>[6x]MFGYFYNSSFRRYATLMGDLFSNIQIKRQ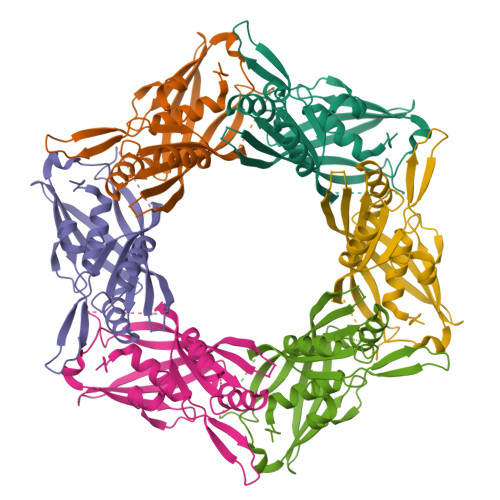LESGDKFIRVPITYASKEHFMMKLNKWTSINSQEDVAKVETILPRINLHLVDFSYNAPFKTNILNQNLLQKGATSVVSQYNPSPIKMIYELSIFTRYEDDMFQIVEQILPYFQPHFNTTMYEQFGNDIPFKRDIKIVLMSAAIDEAIDGDNLSRRRIEWSLTFEVNGWMYPPVDDAEGLIRTTYTDFHANTRDLPDGEGVFESVDSEVVPRDIDPEDWDGTVKQTFTSNVNR2-[(4R)-4-(4-cyanophenyl)-5-ethanoyl-6-methyl-2-oxidanylidene-1-[3-(trifluoromethyl)phenyl]-4H-pyrimidin-3-yl]ethanoic 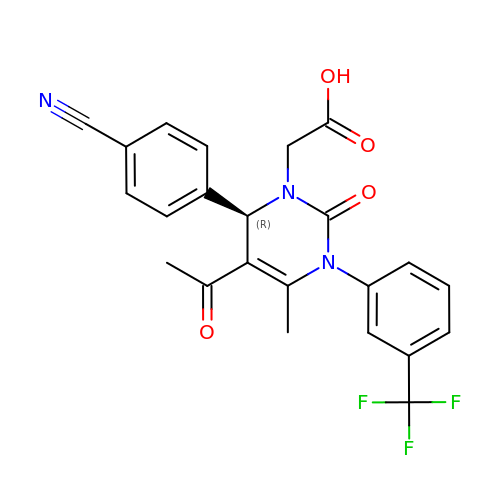acid | C23 H18 F3 N3 O4 | RRKQYMJDNSVFCG-OAQYLSRUSA-N> QQPGEYCHGWVDAQGNYHEGFQCPEDF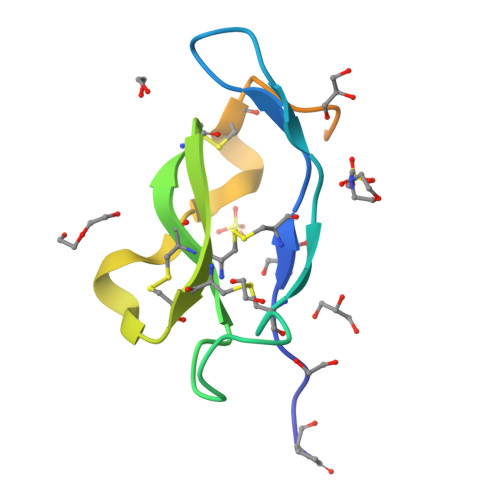DTQDATICCGSCALRYCCAAADARLEQGGCTNDRGELEHPGITAQPVWSHPQFEK As part of our structural genomics effort in targeting novel protein families, we determined crystal structures of three bacterial proteins from a previously structurally uncharacterized protein family Pfam PF08000 [also known as domain of unknown function family 1696 (DUF1696)],11 which appears to be involved in the bacterial cell envelope stress response. These structures share a common domain that is surprisingly similar to the eukaryotic PH-like domains, thus providing the first direct evidence for the existence of PH-like domains in prokaryotes. PHb1 and PHb2 share a common domain that is structurally similar to eukaryotic PH domains, which we have defined as a PHb domain (PH domain in bacteria). The PHb proteins form oligomeric ring assemblies of different sizes and symmetries, providing an excellent example of how molecular architecture can evolve, where the general form of the molecular assembly is preserved, but its size is expandable.

PHb2 contains the PHb domain at its N-terminus (residue 14–136) and a helical-hairpin structure (∼ 68 residues) at the C-terminus that extends out and returns as two α-helices (α1, α2) to the PHb domain. A short helix at the C-terminus (α3) docks between α1 and the β2–β3 (L23) loop and, as a result, links the other end of the hairpin to the PHb domain. This hairpin attachment is crucial for formation of the PHb2 homododecamer. PHb2 is also a dome-shaped assembly, but with C12 cyclic symmetry that is generated by crystallographic C4 axis and a non-crystallographic C3 axis. The PHb2 assembly is significantly larger with an outer diameter of 150 Å, that is, twice that of PHb1(sl). The PHb2 dodecamer buries a total surface area of 46,700 Å2 or ∼ 50% of total surface area (3890 Å2 per monomer). The hairpin constitutes the primary mediator of the central core of the dodecameric PHb2 ring, mainly through hydrophobic interactions. The packing of hairpins involves the docking of surface hydrophobic residues of α1 (around Ile156) and α2 (Val167, Phe171, and Phe179) into a hydrophobic pocket formed by the adjacent hairpin of the neighboring protomer. However, only two main-chain hydrogen bonds [compared to five in PHb1(sl)] are formed between the two strands due to the separation at the N-terminus of β4 and C-terminus of β5 to accommodate the packing of the α1–α2 hairpins. On the other hand, the six independent protomers in the asu of PHb2 have similar packing environment and are essentially identical with each other in structure with an average rmsd of 0.27 Å for 180 aligned Cα atoms.

>[6x]GSDIGQVIHPDDFDKAAADDYVLHEDGEKIYFLIKSKTDEYCFTNLALVHLDGESAVSSKRVLYRYPYAHYPIRHVMFETAGTVDLDVEIKFEIGGKHYSIDVDKKQLEHVKDLYKALLAIAEKQYEGQKMLEFANSSLNHSVTILGGLRQGDMNVPQTFKDLSQESFDWLQGHYYKWNQKDFGSFYEKYINN Apolipoprotein B mRNA-editing enzyme-catalytic polypeptide-like 3G (APOBEC3G or A3G) is a human host restriction factor that inhibits human immunodeficiency virus type 1 (HIV-1), murine leukemia virus, and equine infectious anemia virus primarily through its deoxycytidine deaminase activity on the viral minus-strand DNA (-ssDNA). A3G inhibits viral replication by preferentially deaminating dC to dU in the viral -ssDNA during reverse transcription. Specific “hotspot” sequences of DNA are targeted for deamination, with the highest preference for the 5’-CCCA sequence (where the deaminated C is underlined) in the case of A3G. Extensive biochemical and mutagenesis studies have shown that a single loop, loop 7, of A3G is responsible for selecting the base at the -1 position (the nucleotide at the 5’ side of the deamination site) of the DNA substrate hotspot.

Although A3GCTD overcomes the solubility problem of the full-length protein and retains activity, DNA binding is weak and does not form a stable DNA-protein complex required for structural analysis. To address the problem of weak DNA binding, we designed a novel A3GCTD fusion to protection of telomeres protein 1 (Pot1) from Schizosaccharomyces pombe that serves as an anchor for the DNA (experimental schematic shown in Fig 1A). Using the Pot1A3GCTD fusion construct, we obtained a crystal structure of A3GCTD bound to an adenine nucleotide at 2.9 Å resolution. The structure was determined in a P43 space group with four independent copies of the protein in the asymmetric unit of the crystal. In the crystal, the ssDNA stretches from a Pot1 protein of one fusion complex to the A3G of the adjacent fusion complex. The rest of the ssDNA was disordered with clear electron density for only one nucleotide, adenine, located next to the catalytic site of A3GCTD. In this sequence, the nucleotide preceding the deaminated C is referred to as the -1 nucleotide and the adenine following the deaminated C is the +1 nucleotide. Although we intended to crystallize the A3GCTD bound to its entire hotspot region as described in Fig 1A, we instead captured the A3GCTD bound to a dA in the -1 pocket, which originates from the ssDNA bound to a neighboring Pot1 molecule. In our structure, the adenosine is stabilized by a network of hydrogen bonds and stacking interactions in the -1 pocket. The backbone of residues P210 and I314 hydrogen bond with the amine group of the adenine, while Y315 hydrogen bonds with the phosphate group of the DNA backbone. The adenine base is further stabilized in the pocket through stacking interactions with W211, W285, and Y315. Instead, the A3GCTD -1 pocket accommodates the adenine base by flipping D316 180 degrees away from the nucleotide, which opens the -1 pocket to allow for adenine to bind.

>MVIDSLQLNELLNAGEYKIGELTFQSIRSSQELQKKNTIVNLFGIVKDFTPSRQSLHGTKDWVTTVYLWDPTCDTSSIGLQIHLFSKQGNDLPVIKQVGQPLLLHQITLRSYRDRTQGLSKDQFRYALWPDFSSNSKDTLCPQPMPRLMKTGDKEEQFALLLNKIWDEQTNHSMDPPTFTFNFNNEPWVRGRHETYLCYEVERMHNDTWVKLNQRRGFLANQAPHKHGFLEGRHAELCFLDVIPFWKLDLDQDYRVTCFTSWSPCFSCAQEMAKFISKNKHVSLCIKTARIYDDQGRAQEGLRTLAEAGAKISIMTYSEFKHCWDTFVDHQGAPFQPWDGLDEHSQDLSGRLRAILQNQEN[4x]> MGSHQMKSEEHANMQLQQQAVLGLNWMQDSGEYKALAYQAYNAAKVAFDHAKVAKGKKKAVVADLDETMLDNS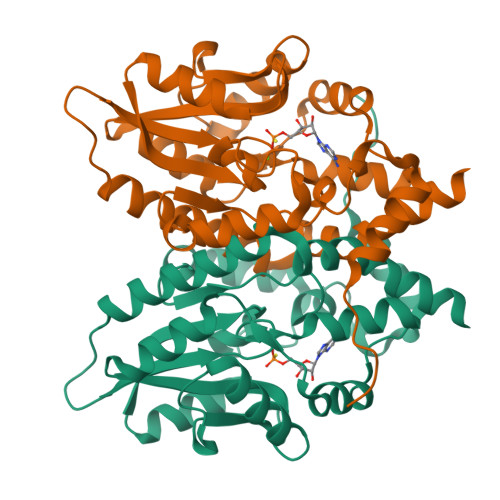PYAGWQVQNNKPFDGKDWTRWVDARQSRAVPGAVEFNNYVNSHNGKVFYVTNRKDSTEKSGTIDDMKRLGFNGVEESAFYLKKDKSAKAARFAEIEKQGYEIVLYVGDNLDDFGNTVYGKLNADRRAFVDQNQGKFGKTFIMLPNANYGGWEGGLAEGYFKKDTQGQIKARLDAVQAWDGKLEHHHHHH> LSNVETEANNIISGNEVGGEIITKVADDASNLLGPNSFATTAQPENKDVVQATTTVNTTNLTQHPSAPTIPFTPDFRNVDNFHSMAYDITTGDKNPSKLIRLDTASWQTSYSRQYKITTVELPKSFWDDTRKPAYGQAKYFAAVRCGFHFQVQVNVNQGTAGSALVVYEPKPVIDSRQYLEFGSLTNLPHVLMNLAETTQADLCIPYVADTNYVKTDSSDLGQLRVYVWTPLSVPTGASNEVDVTVMGS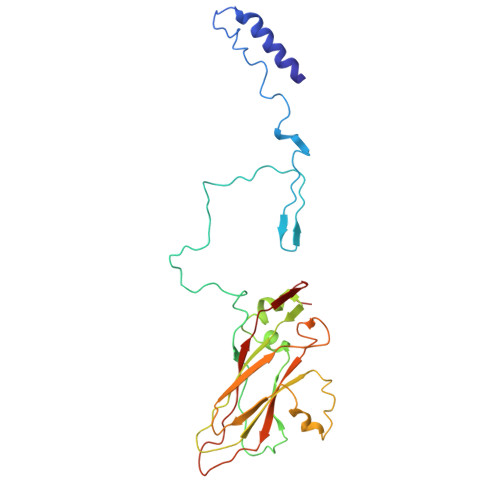LLQLDFQNPRPYGE> SNAMGSVPVELRGDFEVCRRLTRSHYENFSVVSLFVPRHLRPHFYSVYAFCRGVDDLGDEFAGDRMAALDAYEEELRRAFAGEATTPAFRALQFTIATCNLPMEPFLRLIEANRRDQRKHTYD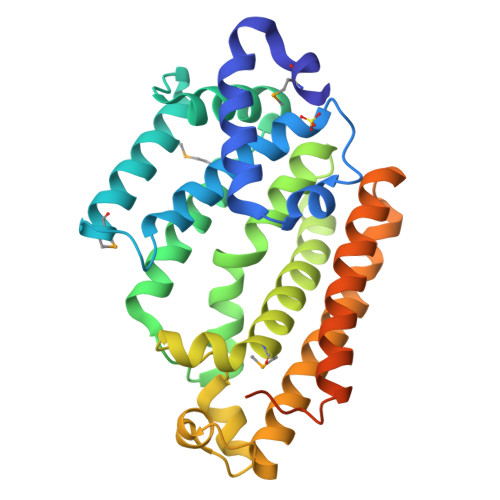TWEDLRDYCRYSADPVGRLVLGIFGCLDDERARLSDATCTALQVANHMQDIDRDLALGRIYVPRADLEQFGATLDDIRARRATDGVRRCIALEVDRAQALFDEGRRLESLVPPRLARQLKLYRLGGEAILAAIRRQGYNPFAGRPVVSGKQKLRIALSVLAGGAKGEGGSA> GSHMASMSKDEVKREAKDTDGNPEIKGERRRLHSEIQSGSLANNIKKSTVIVKN;> PTHIAICLYYKLGETPLPLVIETGKDAKALQIIKLAELYDIPVIEDIPLARSLYKNIHKGQYITEDFFEPVAQLIRIAID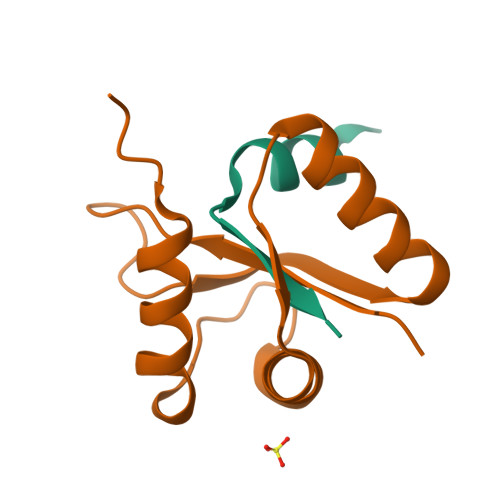LDY>[2x]MSTITRPIIELSNTVDKIAEGNLEAEVPHQNRADEIGILAKSIERLRRSLMRTVGDVRNGANAIYSGASEIATGNNDLSSRTEQQAASLEETAASMEQLTATVKQNAENARQASHLALSASETAQRGGKVVDNVVQTMRDISTSSQKIADIISVIDGIAFQTNILALNAAVEAARAGEQGRGFAVVAGEVRNLA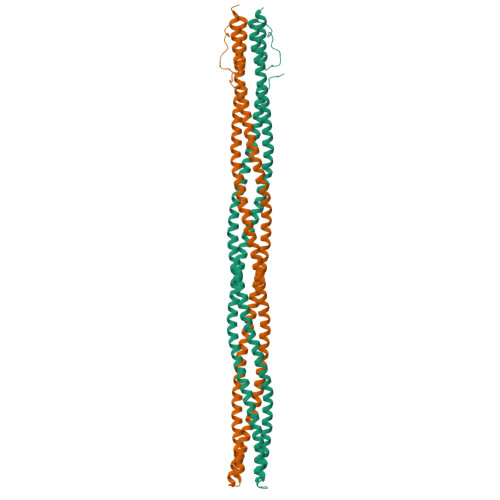QRSAQAAREIKSLIEDSVGKVDVGSTLVESAGETMAEIVSAVTRVTDIMGEIASASDEQSRGIDQVGLAVAEMDRVTQQNAALVEESAAAAAALEEQASRLTEAVAVFRIQQQQQQQRETSAVVKTVTPATPRKMAVADSGENWETF> MKEFYLTVEQIGDSIFERYIDSNGRERTREVEYKPSLFAHCPESQATKYFDIYGKPCTRKLFANMRDASQWIKRMEDIGLEALGMDDFKLAYLSDTYNYEIKYDHTKIRVANFDIEVTSPDGFPEPSQAKHPIDAITHYDSIDDRFYVFDLLNSPYGNVEEWSIEIAAKLQEQGGDEVPSEIIDKIIYMPFDNEKELLMEYLNFWQQKTPVILTGWNVESFAIPYVYNRIKNIF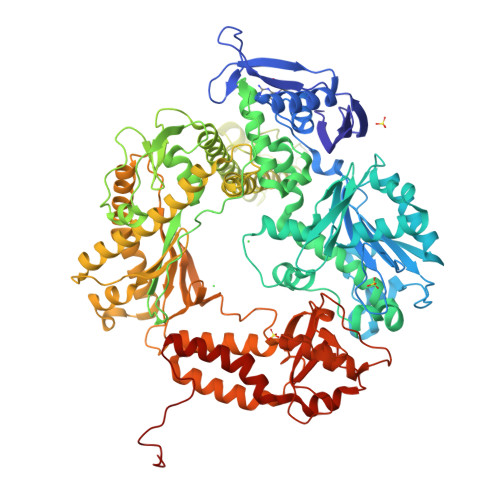GESTAKRLSPHRKTRVKVIENMYGSREIITLFGISVLDYIDLYKKFSFTNQPSYSLDYISEFELNVGKLKYDGPISKLRESNHQRYISYNIIAVYRVLQIDAKRQFINLSLDMGYYAKIQIQSVFSPIKTWDAIIFNSLKEQNKVIPQGRSHPVQPYPGAFVKEPIPNRYKYVMSFDLTSLYPSIIRQVNISPETIAGTFKVAPLHDYINAVAERPSDVYSCSPNGMMYYKDRDGVVPTEITKVFNQRKEHKGYMLAAQRNGEIIKEALHNPNLSVDEPLDVDYRFDFSDEIKEKIKKLSAKSLNEMLFRAQRTEVAGMTAQINRKLLINSLYGALGNVWFRYYDLRNATAITTFGQMALQWIERKVNEYLNEVCGTEGEAFVLYGDTDSIYVSADKIIDKVGESKFRDTNHWVDFLDKFARERMEPAIDRGFREMCEYMNNKQHLMFMDREAIAGPPLGSKGIGGFWTGKKRYALNVWAMEGTRYAEPKLKIMGLETQKSSTPKAVQKALKECIRRMLQEGEESLQEYFKEFEKEFRQLNYISIASVSSANNIAKYDVGGFPGPKCPFHIRGILTYNRAIKGNIDAPQVVEGEKVYVLPLREGNPFGDKCIAWPSGTEITDLIKDDVLHWMDYTVLLEKTFIKPLEGFTSAAKLDYEKKASLFDMFDF>[8x]GPMPQLTLD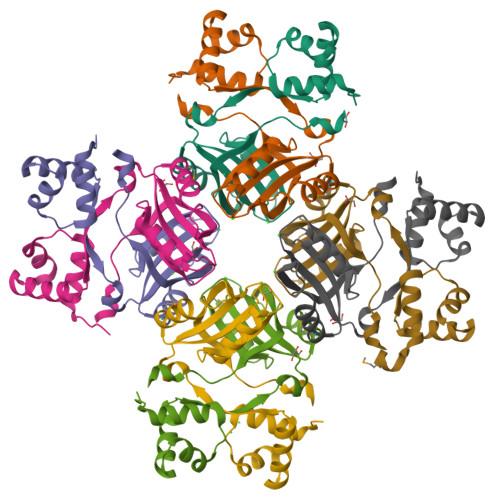KTDIKILQVLQENGRLTNVELSERVALSPSPCLRRLKQLEDAGIVRQYAALLSPESVNLGLQAFIRVSIRKAKDAREDFAASVRKWPEVLSCFALTGETDYLLQAFFTDMNAFSHFVLDTLLSHHGVQDAQSSFVLKEIKHTTSLPLNHLLKE> MRGSHHHHHHTDPQGDAAQKTDTSHHDQDHPTFNKITPNLAEFAFSLYRQLAHQSNSTNIFFSPVSIATAFAMLSLGTKADTHDEILE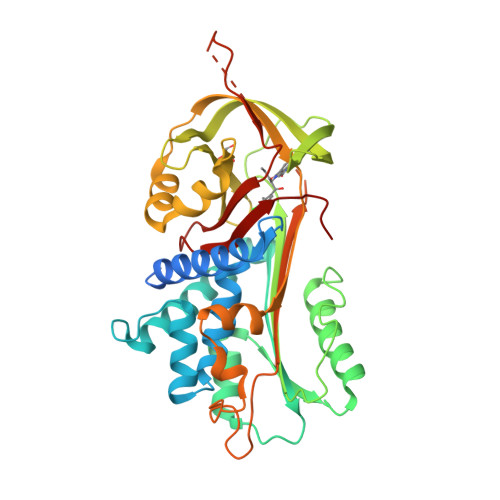GLNFNLTEIPEAQIHEGFQELLRTLNQPDSQLQLTTGNGLFLSEGLKLVDKFLEDVKKLYHSEAFTVNFGDTEEAKKQINDYVEKGTQGKIVDLVKELDRDTVFALVNYIFFKGKWERPFEVKDTEEEDFHVDQVTTVKVPMMKRLGMFNIQHSKKLSSWVLLMKYLGNATAIFFLPDEGKLQHLENELTHDIITKFLENEDRRSASLHLPKLSITGTYDLKSVLGQLGITKVFSNGADLSGVTEEAPLKLSKAVHKAVLTIDEKGTEAAGAMFLEAIPMSIPPEVKFNKPFVFLMIEQNTKSPLFMGKVVNPTQK>[5x]LDRADILYNIRQTSRPDVIPTQRDRPVAVSVSLKFINILEVNEITNEVDVVFWQQTTWSDRTLAWNSSHSPDQVSVPISSLWVPDLAAYNAISKPEVLTPQLARVVSDGEV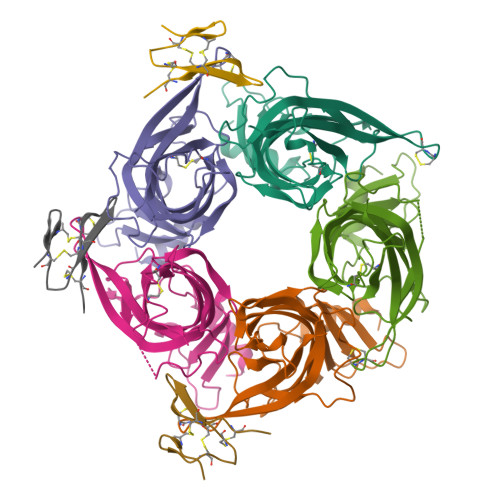LYMPSIRQRFSCDVSGVDTESGATCRIKIGSWTHHSREISVDPTTENSDDSEYFSQYSRFEILDVTQKKNSVTYSCCPEAYEDVEVSLNFRKKG;>[3x]TRMCGSMSCPRNGCTCVYHWRRGHGCSCPG> ADYDLKF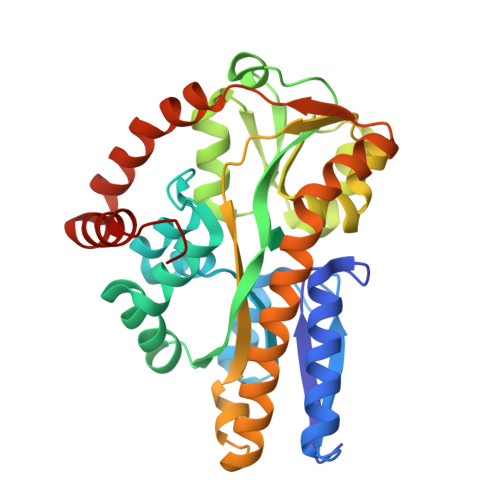GMNAGTSSNEYKAAEMFAKEVKEKSQGKIEISLYPSSQLGDDRAMLKQLKDGSLDFTFAESARFQLFYPEAAVFALPYVISNYNVAQKALFDTEFGKDLIKKMDKDLGVTLLSQAYNGTRQTTSNRAINSIADMKGLKLRVPNAATNLAYAKYVGASPTPMAFSEVYLALQTNAVDGQENPLAAVQAQKFYEVQKFLAMTNHILNDQLYLVSNETYKELPEDLQKVVKDAAENAAKYHTKLFVDGEKDLVTFFEKQGVKITHPDLVPFKESMKPYYAEFVKQTGQKGESALKQIEAINPHHH>[2x]MDFGSLETVVANSAFIAARGSFDASSGPASRDRKYLARLKLPPLSKCEALRESLDLGFEGMCLEQPIGKRLFQQFLRTHEQHGPALQLWKDIEDYDTADDALRPQKAQALRAAYLEPQAQLFCSFLDAETVARARAGAGDGLFQPLLRAVLAHLGQAPFQEFLDSLYFLRFLQWKWLEAQPMGEDWFLDFRVLGRGGFGEVFACQMKATGKLYACKKLNKKRLKKRKGYQGAMVEKKILAKVHSRFIVSLAYAFETKTDLCLVMTIMNGGDIRYHIYNVDEDNPGFQEPRAIFYTAQIVSGLEHLHQRNIIYRDLKPENVLLDDDGNVRISDLGLAVELKAGQTKTKGYAGTPGFMAPELLLGEEYDFSVDYFALGVTLYEMIAARGPFRARGEKVENKELKQRVLEQAVTYPDKFSPASKDFCEALLQKDPEKRLGFRDGSCDGLRTHPLFRDISWRQLEAGMLTPPFVPDSRTVYAKNIQ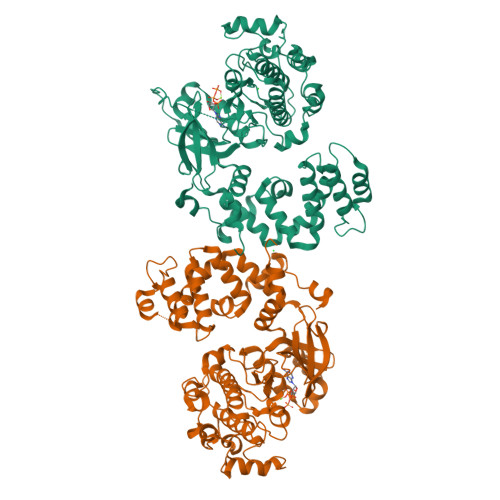DVGAFSTVKGVAFEKADTEFFQEFASGTCPIPWQEEMIETGVFGDLNVWRPDGVDHHHHHH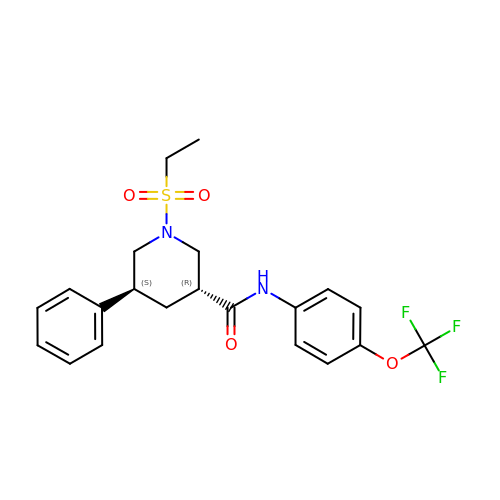(3R,5S)-1-(ethanesulfonyl)-5-phenyl-N-[4-(trifluoromethoxy)phenyl]piperidine-3-carboxamide (bound form) | C21 H23 F3 N2 O4 S | BGPUEQUEKKTRNM-IAGOWNOFSA-N> GPGSMEASCLELALEGERLCKSGDCRAGVSFFEAAVQVGTEDLKTLSAIYSQLGNAYFYLHDYAKALEYHHHDLTLARTIGDQLGEAKASGNLGNTLKVLGNFDEAIVCCQRHLDISRELNDKVGEARALYNLGNVYHAKGKSFGCPGPQDVGEFPEEVRDALQAAVDFYEENLSLVTALGDRAAQGRAFGNLGNTHYLLGNFRDAVIAHEQRLLIAKEFGDKAAERRAYSNLGNAYIFLGEFETASEYYKKTLLLARQLKDRAVEAQSCYSLGNTYTLLQDYEKAIDYHLKHLAIAQELNDRIGEGRACWSLGNAYTALGNHDQAMHFAEKHLEISREVGDKSGELTARLNLSDLQMVLGLSYSTNNSIMSENT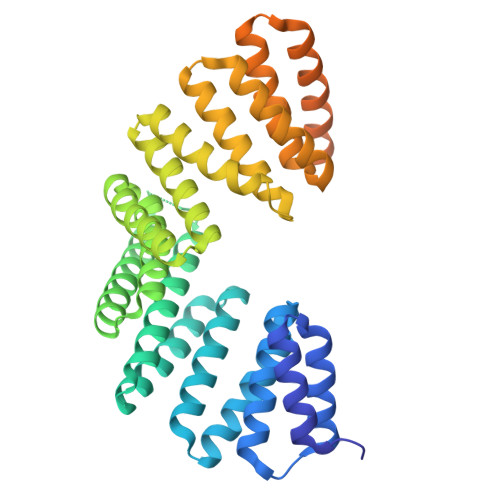EIDSSLNGVRPKLGRRHSMENMELMKLTPEK> QGHMSNFLAEQYERDRKAIINCCFSRPDHKTGEPPNNYITHVRIIEDSKFPSSRPPPDSKLENKKKRLLILSAKPNNAKLIQIHKARENSDGSFQIGRTWQLTELVRVEKDLEISEGFILTMSKKYYWETNSAKERTVFIKSLITLYIQTFEGHVPELVNWDLSLFYLDERSYQRAVITNRPGSVSPIKSPTSNFTTNTTQSVGSVPFSAPTE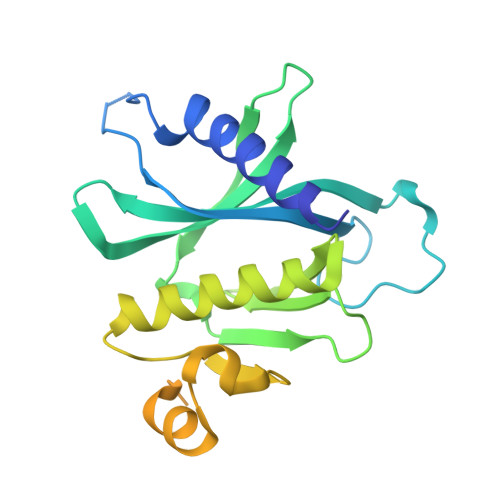RTRRSETESVNPVSTPASVEYHAGMKSLNKAPYSSNS>[4x]GIDPFTKMTRPSSDLTAFREHFAKAKHIAIITGAGVSAESGVPTFRGPGGFWRKWQAQDLATPEAFSRDPSLVWEFYHYRREVMRSKMPNPAHLAIAECEARLGQQGRSVVIITQNIDELHHRAGSKHVYEIHGSLFKTRCMSCGEVKANHKSPICPALDGKGAPDPNTKEARIPVELLPRCERKSCNG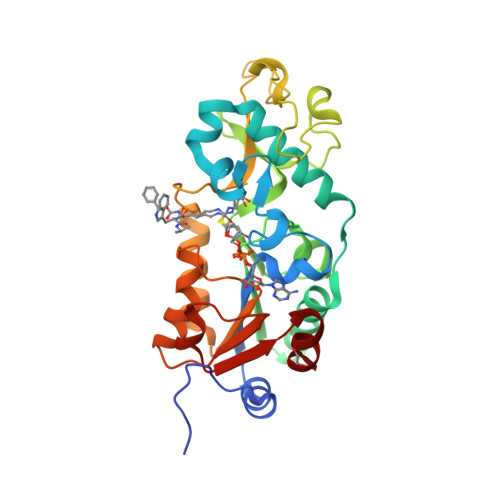LLRPHVVWFGETLDSDILTAVERELEKCDLCLVVGTSSIVYPAAMFAPQVASRGVPVAEFNMECTPATQRFKYHFEGPCGSTLPPALE>[2x]MEEPEEPADSGQSLVPVYIYSPEYVSMCDSLAKIPKRADMVHSLIEAYALHKQMRIVKPKVASMEEMATFHTDAYLQHLQKVSQEGDDDHPDSIEYGLGYDCPATEGIFDYAAAIGGATITAAQCLIDGMCKVAINWSGGWHHAKKDEASGFCYLNDAVLGILRLRRKFERILYVDLDLHHGDGVEDAFSFTSKVMTVSLHKFSPGFFPGTGDVSDVG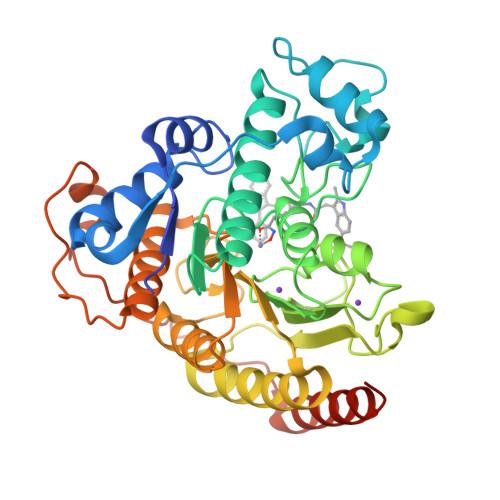LGKGRYYSVNVPIQDGIQDEKYYQICESVLKEVYQAFNPKAVVLQLGADTIAGDPMCSFNMTPVGIGKCLKYILQWQLATLILGGGGYNLANTARCWTYLTGVILGKTLSSEIPDHEFFTAYGPDYVLEITPSCRPDRNEPHRIQQILNYIKGNLKHVVIEGRSHHHHHH> GSHMLETFNKITPNLAEFAFSLYRQLAHQSNSTNIFFSPVSIATAFAMLSLGTKADTHDEILEGLNFNLTEIPEAQIHEGFQELLRTLNQPDSQLQLTTGNGLFLSEGLKLVDKFLEDVKKLYHSEAFTVNFGDTEEAKKQINDYVEKGTQGKIVDLVKELDRDTVFALVNYIFFKGKWERPFEVKDTEEEDFHVDQVTTVKVPMMKRLGMFNIQHAKKLSSWVLLMKYLGNATAIFFLPDEGKLQHLENELTHDIITKFLENEDRRSASLHLPKLSITGTYDLKSVLGQLGI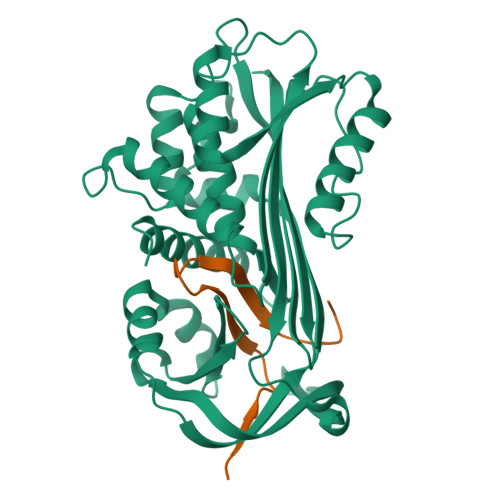TKVFSNGADLSGVTEEAPLKLSKAVHKAVLTIDEKGTEAAGADDDEAIPR;> SIPPEVKFNKPFVFLMIEQNTKSPLFMGKVVNPTQK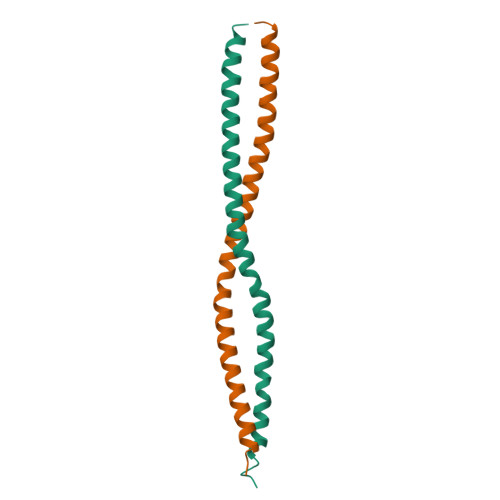>[2x]GSGMQLEDLRQQLQQAEEALVAKQELIDKLKEEAEQHNIVMETVPVLKAQADIYKADFQAERHAREKLVEKKEYLQEQLEQLQREFNKLKVG>[2x]AEAGITGTWYNQLGST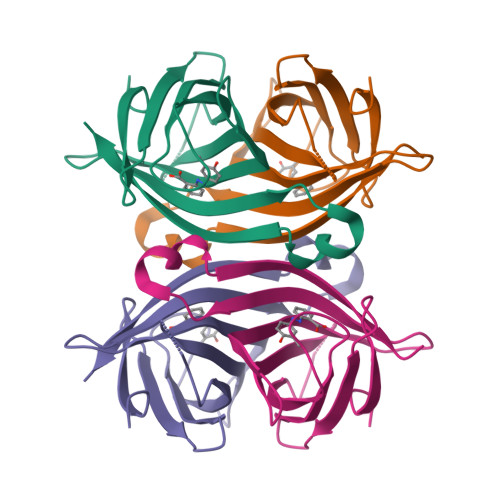FIVTAGADGALTGTYESAVGNAESRYVLTGRYDSAPATDGSGTALGWTVAWKNNYRNAHSATTWSGQYVGGAEARINTQWLLTSGTTEANAWKSTLVGHDTFTKV>MFGRKKGDVIDAGAELERAEQERIEGEYGASELASERRPHTPGARTLLMVLLCVIAVVLVTLSYKAYKVRGVVEDDDAQPQQVVRQVIPGYTPRPIRPEPENVPEPPQPTTSVPAIQPAPVTQPVRPQPTGPREKTPYELARERMLRSGLTAGSGGGEDLPRPQGGDVPAGGLMGGGGGGGELAEKLQPMRLSGSSAGRLGNRDMLITQGTQLDCVLETRLVTTQPGMTTCHLTRDVYSTSGRVVLLDRGSKVVGFYQGGLRQGQARIFVQWSRIETPSGVVINLDSPGTGPLGEAGLGGWIDRHFWERFGGAIMISLIGDLGDWASRQGSRQGDNSIQFSNTANGVESAAAEALRNSINIPPTLYKNQGERVNILVARDLDFSDVYSLESIPTK[16x];>MKKLAIVALLASLHAVPALALDVPSSSRYDHRIRYVTYNPADVVQVDTVLGVATHIMLEEGEQYLTHAFGDSEAYAFARKGRHIFIKPQAELANTNLIVVTDRRSYKFRLQMRNDRNGAMYELAFRYPDTQARQTREANARAAVEAAFEQRVGAYYNLKYMMSGDKDIAPVNAWDDGRFTYFKFSANADLPSIYFVDAEGNESLVPRTTVGSSNNIIAVHKVNPKWMIRLGNRALAIFNEAYD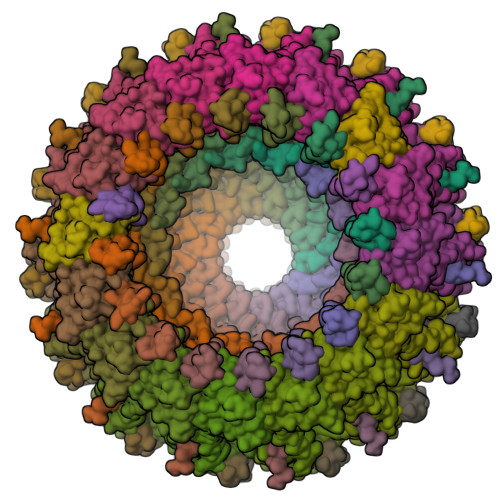PNGVPNDTGTASPAVRRVNKGGN[16x];>MKTIIFAILMTGLLSACASAPKPKQPSDFNREPVNKTVPVEIQRGAL[14x]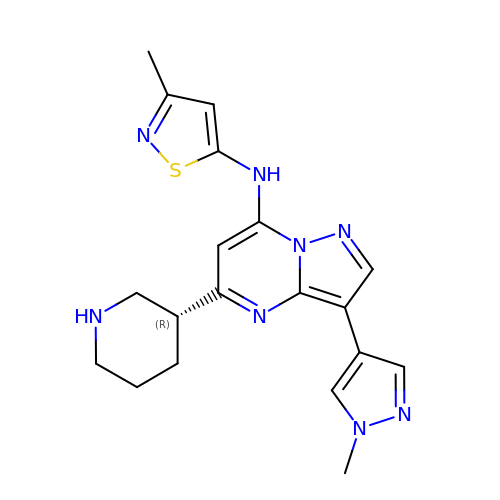N-(3-methylisothiazol-5-yl)-3-(1-methyl-1H-pyrazol-4-yl)-5-[(3R)-piperidin-3-yl]pyrazolo[1,5-a]pyrimidin-7-amine | C19 H22 N8 S | GZPYWHILDNLCNY-CYBMUJFWSA-N3-CHLORO-N-(4-CHLORO-2-{[(5-CHLOROPYRIDIN-2-YL)AMINO]CARBONYL}-6-METHOXYPHENYL)-4-[(1-METHYL-1H-IMIDAZOL-2-YL)METHYL]THIOPHENE-2-CARBOXAMIDE | C23 H18 Cl3 N5 O3 S | 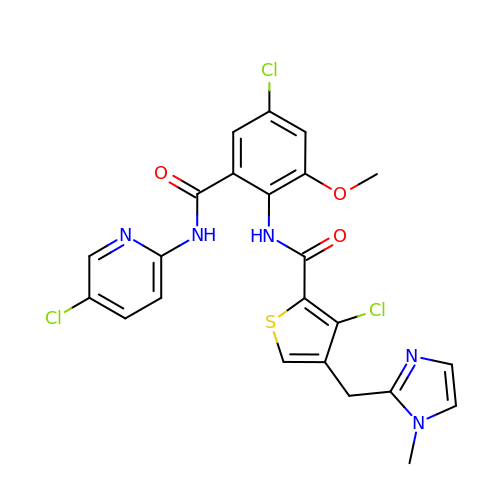WBFPCLIRIGEEBD-UHFFFAOYSA-N> MRRYEVNIVLNPNLDQSQLALEKEIIQRALENYGARVEKVEELGLRRLAYPIAKDPQGYFLWYQVEMPEDRVNDLARE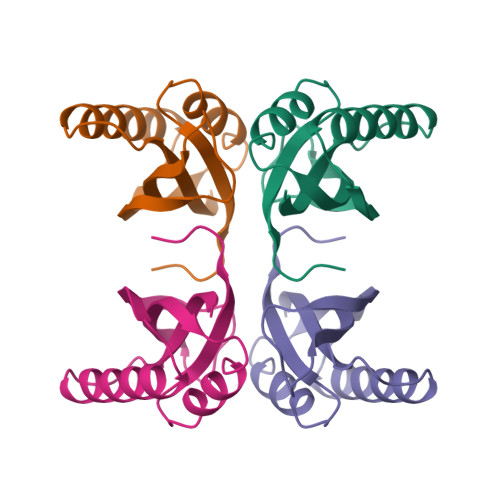LRIRDNVRRVMVVKSQEPFLANA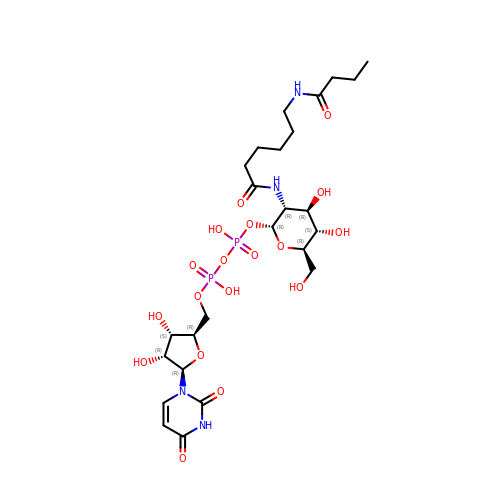[[(2~{R},3~{S},4~{R},5~{R})-5-[2,4-bis(oxidanylidene)pyrimidin-1-yl]-3,4-bis(oxidanyl)oxolan-2-yl]methoxy-oxidanyl-phosphoryl] [(2~{R},3~{R},4~{R},5~{S},6~{R})-3-[6-(butanoylamino)hexanoylamino]-6-(hydroxymethyl)-4,5-bis(oxidanyl)oxan-2-yl] hydrogen phosphate | C25 H42 N4 O18 P2 | MGZXRAPGBJHSCZ-HDEQREAESA-N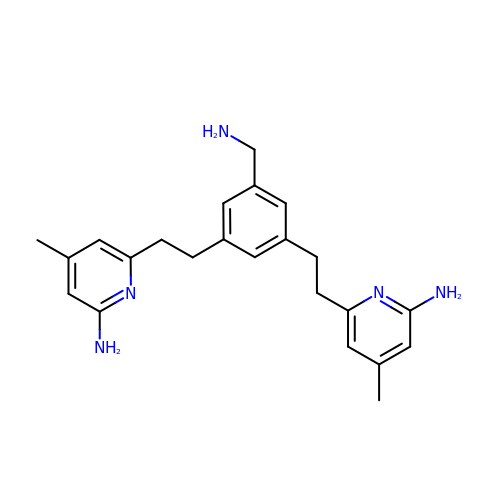6,6'-{[5-(aminomethyl)benzene-1,3-diyl]diethane-2,1-diyl}bis(4-methylpyridin-2-amine) | C23 H29 N5 | JCCJTHWRJDOXTL-UHFFFAOYSA-N> GPGFDFAQAIMKKNTVVARTEKGEFTMLGVHDRVAVIPTHASVGETIYINDVETKVLDACALRDLTDTNLEITIVKLDRNQKFRDIRHFLPRYEDDYNDAVLSVHTSKFPNMYIPVGQVTNYGFLNLGGTPTHRILMYNFPTRAGQCGGVVTTTGKVIGIHVGGNGAQGFAAMLLHSYFTDTQKHHHHHH

The Picornaviridae family of single-stranded, positive-sense, non-enveloped RNA viruses includes several pathogens of concern such as enterovirus-D68 (EV68). The 3C protease cleaves eight sites within the viral polyprotein, with a preference for a glutamine–glycine (QG) motif at the P1/P1′ positions, a preference distinct from host cysteine proteases. Among strains of EV68, the amino acid sequences of 3C protease and its cleavage sites are highly conserved. We have determined and analyzed three high-resolution inhibitor-bound crystal structures of EV68-3C protease, which revealed possible sites of resistance mutations, a key structural water molecule conserved during ligand binding, and the conformational flexibility of the catalytic histidine H40.

Rupintrivir demonstrated the highest potency with the IC50 value in the single-digit nanomolar range, followed closely by AG7404. From these data, the shared scaffold of rupintrivir/AG7404 appears to be well accommodated within the active site of EV68-3C protease. Within the active site, rupintrivir and AG7404 exhibited identical hydrogen bonds from P4 to P1′, with one additional hydrogen bond formed between AG7404 and C147 backbone nitrogen. The observed conformational flexibility of His40 was likely due to differences between inhibitor P2 moieties. At P2, AG7404 lacked the fluorinated phenylalanine ring of rupintrivir and was unable to pi-stack on the catalytic His40. As AG7404 is an analog of rupintrivir, this compound shares many structural similarities and protrudes in the same regions, highlighted at the S4 pocket, where the isoxazole ring forms the same hydrogen bond contact with Asn165. At the S4 pocket, the mutation of Asn165 into a larger residue could preclude binding of the inhibitors, while other mutations could remove the potential for hydrogen bond formation, potentially decreasing inhibitor binding. Furthermore, this additional hydrogen bond formation, not conserved in viral substrate interactions, has been implicated in resistance against rupintrivir in HRV-3C protease. While there are no sequences of circulating strains with mutations at these residues, mutations can emergence under repeat exposure to inhibitors. This concern is exemplified by previous studies that demonstrated a 7-fold (V104I) and 15-fold (N165T, A103V, and E3G) decrease in potency when mutations arise in HRV-3C protease against rupintrivir. From our structural analysis, we predict that EV68 strains with similar mutations would likely demonstrate some level of resistance toward these inhibitors.> EQSSSEIKIVRDEYGMPHIYANDTWHLFYGYGYVVAQDRLFQMEMARRSTQGTVAEVLGKDFVKFDKDIRRNYWPDAIRAQIAALSPEDMSILQGYADGMNAWIDKVNTNPETLLPKQFNTFGFTPKRWEPFDVAMIFVGTMANRFSDSTSEIDNLALLTALKDKYGVSQGMAVFNQLKWLVNPSAPTTIAVQESNYPLKFNQQNSQTA;> SNMWVIGKSKAQDAKAIMVNGPQFGWYAPAYTYGIGLHGAGYDVTGNTPFAYPGLVFGHNGVISWGSTAGLGDDVDIFAERLSAEKPGYYLHNGKWVKMLSREETITVKNGQAETFTVWRTVHGNILQTDQTTQTAYAKSRAWDGKEVASLLAWTHQMKAKNWQEWTQQAAKQALTINWYYADVNGNIGYVHTGAYPDRQSGHDPRLPVPGTGKWDWKGLLPFEMNPKVYNPQSGYIANWNNSPQKDYPASDLFAFLWGGADRVTEIDRLLEQKPRLTADQAWDVIRQTSRQDLNLRLFLPTLQAATSGLTQSDPRRQLVETLTRWDGINLLNDDGKTWQQPGSAILNVWLTSMLKRTVVAAVPMPFDKWYSASGYETTQDGPTGSLNISVGAKILYEAVQGDKSPIPQAVDLFAGKPQQEVVLAALEDTWETLSKRYGN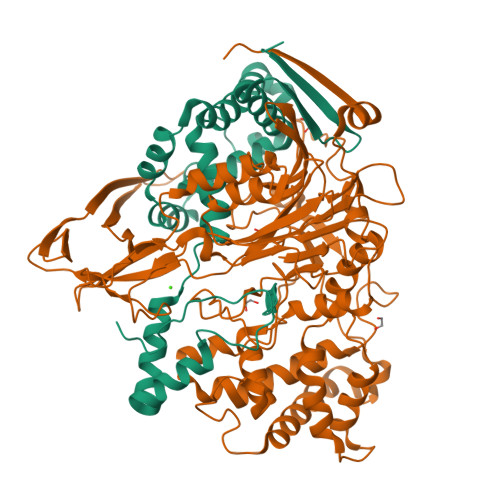NVSNWKTPAMALTFRANNFFGVPQAAAEETRHQAEYQNRGTENDMIVFSPTTSDRPVLAWDVVAPGQSGFIAPDGTVDKHYEDQLKMYENFGRKSLWLTKQDVEAHKESQEVLHVQR Glutathionyl-hydroquinone reductases (GHRs) belong to the glutathione transferase (GST) family of enzymes and catalyze efficiently the reduction of hydrophobic, bulky glutathionyl-hydroquinones. One of the most studied GHRs from a biochemical point of view is the protein ECM4 from the yeast Saccharomyces cerevisiae (ScECM4). In this study, we described the X-ray structures of ScECM4 and glutathionylated ScECM4 (ScECM4-SG). Besides the features that defined these GSTs as members of the class Xi, ScECM4 possessed a tremendously elongated loop between strand β2 and helix α2 involved in the dimer interface, two more spiral turns in helix α5 that make it 45 Å long and an additional helix α5’ with two helical turns.

Crystallization of ScECM4 was assayed by the microbatch under paraffin oil method at 278 K. ScECM4 (41 mg/mL) crystallized by mixing 1 μL of protein with 1 μL of commercial crystallization solution (Wizard I n°10 (Rigaku), consisting of 20% (w/v) polyethyleneglycol 2000 monomethylether in 0.1 M Tris-HCl buffer, pH 7.0). ScECM4 and ScECM4-SG crystals diffracted respectively to 1.45 Å and 1.68 Å according to the CC1/2 correlation coefficient. ScECM4 exhibited no GSH in the active site but rather glycerol molecules. As expected, the monomer of ScECM4 exhibited the GST fold and dimerized with the pattern specific to GSTXs. The N-terminal domain (G11-K196) adopted the thioredoxin fold (β1α1β2α2β3β4α3) and the C-terminal domain (K197-E372) was found to be all helical (α4α5α5’α6α7α8α9). The typical features of GSTXs were also present: a long N-terminal end (37-residues), an extended loop between β2 and α2 (V70-R140) and a unique dimerization mode by the helical domain. The visible N-terminal end starting from G11 was found to be partially surrounding the active site in ScECM4 and in monomer A of ScECM4-SG. G11 was hydrogen-bonded with E230, at the C-terminal end of helix α4. The loop β2-α2 (residues V70-R140) was the second distinctiveness of ScECM4, and probably the most striking one. The side chain of S115 and the main chain of A117 were hydrogen-bonded to the side chain of E236 in the helix α5 of the other monomer.

>[2x]MSKQWASGTNGAFKRQVSSFRETISKQHPIYKPAKGRYWLYVSLACPWAHRTLITRALKGLTSVIGCSVVHWHLDEKGWRFLDMEKQLEDSEDFLEHWHDVAGGIRTAKEDSSKSFAEIKNDSQRFMVDATNEPHYGYKRISDLYYKSDPQYSARFTVPVLWDLETQTIVNNESSEIIRILNSSAFDEFVDDDHKKTDLVPAQLKTQIDDFNSWVYDSINNGVYKTGFAEKAEVYESEVNNVFEHLDKVEKILSDKYSKLKAKYGEEDRQKILGEFFTVGDQLTEADIRLYTTVIRFDPVYVQHFKCNFTSIRAGYPFIHLWVRNLYWNYDAFRYTTDFDHIKLHYTRSHTRINPLGITPLGPKPDIRPLLEHHHHHH>[4x]SNAMRTQVSREPFGTLDDGTRVDRWTLESGPAGLRVRVLTYGGIVQTVEAPDRDGMRGQLALGFADLASYAAHGGSYFGALVGRYANRIAGASFVLDGRTDALTPNNGRHSLHGGPGGFSRVVWDAREVDGGVQLHRVSPDGEEGFPGALDVRVTYTLSAGALRIVSCATTDAPTVVNLTNHTYLNLGGDGSGSAAGHELRLAAS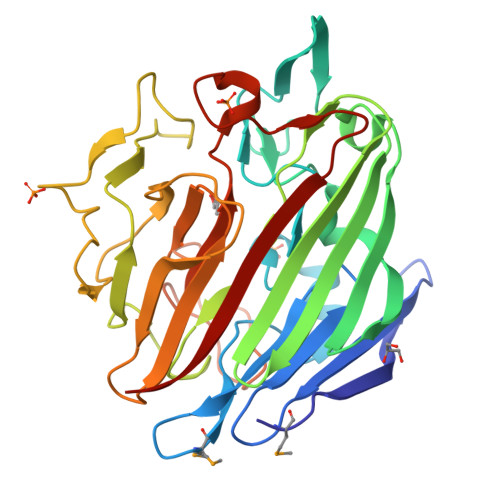RYTPVDGTGIPVPGAPAEVTGTRFDFRAARAVAGAYDHNFALDGGVREAPRTVAELYDPRSGRALALATTEPGLQLYTADHLDGTLTGTSGVPYGPAAGLALETQHFPDSPNRPDFPSTVLRPGESYRSETVYAFSVR> MGSSHHHHHHSSGRENLYFQGHMEKDRKRILITGGAGFVGSHLTDKLMMDGHEVTVVDNFFTGRKRNVEHWIGHENFELINHDVVEPLYIEVDQIYHLASPASPPNYMYNPIKTLKTNTIGTLNMLGLAKRVGARLLLASTSEVYGDPEVHPQSEDYWGHVNPIGPRACYDEGKRVAETMCYAY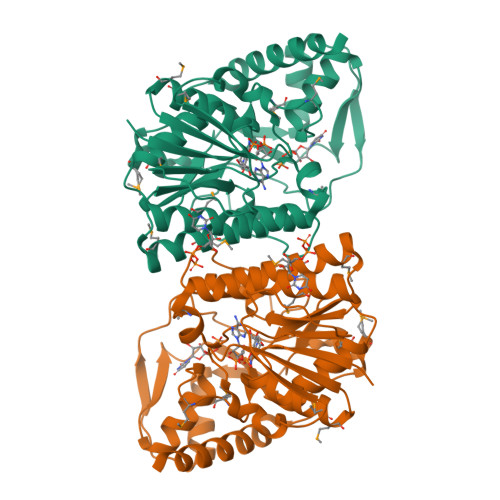MKQEGVEVRVARIFNTFGPRMHMNDGRVVSNFILQALQGEPLTVYGSGSQTRAFQYVSDLVNGLVALMNSNVSSPVNLGNPEEHTILEFAQLIKNLVGSGSEIQFLSEAQDDPQKRKPDIKKAKLMLGWEPVVPLEEGLNKAIHYFRKELEYQANNQGS To investigate the architectural parameters that dictate the substrate specificity and site-selectivity of a Rieske oxygenase catalyzed reaction, we focused on two Rieske oxygenases, SxtT and GxtA, which are involved in the biosynthesis of paralytic shellfish toxins. These enzymes share 88% sequence identity with one another and selectively install a hydroxyl group on adjacent C12 and C11 positions of a tricyclic saxitoxin scaffold, respectively. Each structure showcases an α3 trimeric architecture, and each protomer of the trimer contains a Rieske cluster in the N-terminal domain and a non-heme iron center in the C-terminal domain. The trimeric quaternary architecture places these metallocenters within electron transfer distance of one another across the subunit-subunit interfaces.

To investigate how the native hydroxylated substrates bind to SxtT and GxtA and to identify global architectural differences between these proteins, we solved the structures of SxtT and GxtA with β-STOH bound, as well as that of GxtA with STX, bound to 1.79-, 1.79-, and 1.74-Å resolution, respectively. In GxtA, STX also forms extra active-site interactions. Here, the addition of a hydroxyl group at the C12 α-position allows for the formation of hydrogen bonds with Ser159 and Tyr255, explaining the previously noted structural importance of Tyr255 for selectivity. The remaining GxtA interactions are formed between β-STOH and STX with Asp239 and Gln226. In GxtA, there are only two recognition points for the native STX substrate. Gln226 and Asp239 interact with the guanidinium of the five-membered ring of ddSTX, β-STOH, and STX, and Tyr255 interacts with the α-hydroxyl group of STX, which is installed by SxtT. The most significant structural difference between these substrate-bound structures of SxtT and GxtA is the orientation of a loop that connects the β13 and β14 strands of the C-terminal iron-binding domain. In contrast, the two-loop orientations in GxtA extend away from the active site.

>MTTADLILINNWYVVAKVEDCRPGSITTAHLLGVKLVLWRSHEQNSPIQVWQDYCPHRGVPLSMGEVANNTLVCPYHGWRYNQAGKCVQIPAHPDMVPPASAQAKTYHCQERYGLVWVCLGNPVNDIPSFPEWDDPNYHKTYTKSYLIQASPFRVMDNSIDVSHFPFIHEGILGDRNHAEVEDLEVKVDKDGLTMGKYQVHTSKFNNSTKDDSMVNWFRLSHPLCQYCSTEASEMRTVDLMVVTPIDEDNSVLRYLIMWNGSKTLESKILADYDQVIEEDIRILHSQQPTRLPLLSPKQINTQGLPQEIHVPSDRCTVAYRRWLKELGVTYGVC[3x]> MANQRMLGFVHTAQRMPDKRPAAERRQDFAEIYARFSDERANEQANRCSQCGVPFCQVHCPVSNNIPDWLKLTSEGRLE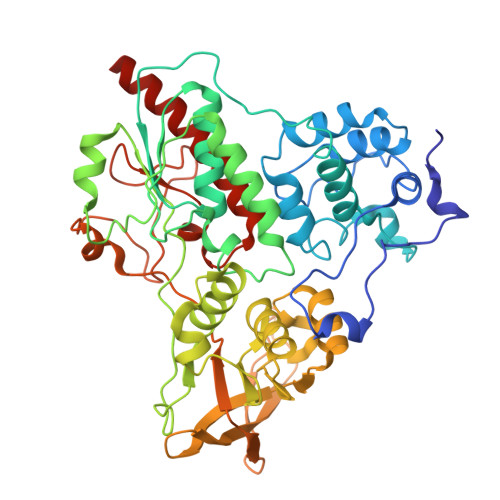EAYEVSQATNNFPEICGRICPQDRLCEGNCVIEQSTHGAVTIGSVEKYINDTAWDQGWVKPRTPSRELGLSVGVIGAGPAGLAAAEELRAKGYEVHVYDRYDRMGGLLVYGIPGFKLEKSVVERRVKLLADAGVIYHPNFEVGRDASLPELRRKHVAVLVATGVYKARDIKAPGSGLGNIVAALDYLTTSNKVSLGDTVEAYENGSLNAAGKHVVVLGGGDTAMDCVRTAIRQGATSVKCLYRRDRKNMPGSQREVAHAEEEGVEFIWQAAPEGFTGDTVVTGVRAVRIHLGVADATGRQTPQVIEGSEFTVQADLVIKALGFEPEDLPNAFDEPELKVTRWGTLLVDHRTKMTNMDGVFAAGDIVRGASLVVWAIRDGRDAAEGIHAYAKAKAEAPVAVAAE> LNPQLVQPAKKPYNKIVSHLLVAEPEKIYAMPDPTVPDSDIKALTTLCDLADRELVVIIGWAKHIPGFSTLSLADQMSLLQSAWMEILILGVVYRSLSFEDELVYADDYIMDEDQSKLAGLLDLNNAILQLVKKYKSMKLEKEEFVTLKAIALANSDSMHIEDVEAVQKLQDVLHEALQDYEAGQHMEDPRRAGKMLMTLPLLRQ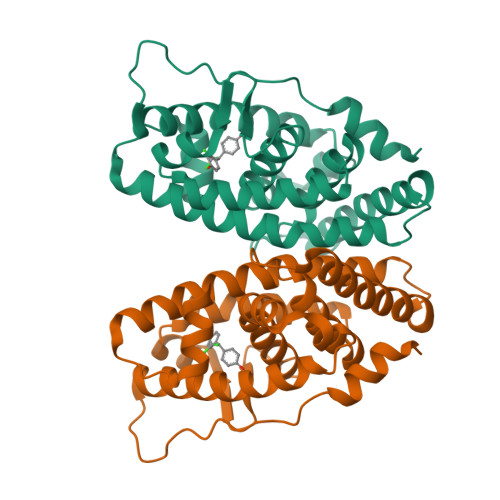TSTKAVQHFYNIKLEGKVPMHKLFLEMLEAKV> GMQKDSKIYIAGHSGLVGSAILNELKQQGYKNLVFKTHFELDLTNQKAVADFFEREKPEYVILAAAKAGGILANNTYRADFIYQNLMIECNVIHNAYLHKVKKLLFIASTTVYPKNATLPTSEEQMLSGDLEYTNKPYAIAKISGLMLCESYNLQYNTNFIAITPTNLYGNNDKFDLEKSHVLPGILRKMHLAKLLNEKRYEDLLNDLKFDSIEEAKNYLKKFGVDKDNVEIWGSGKPTREFLHSQDLANACLFIMNNIDFKDLKSDNIEIINTHLNIGPHKNITIKELAELIKNIVGFKGKLVFNLNR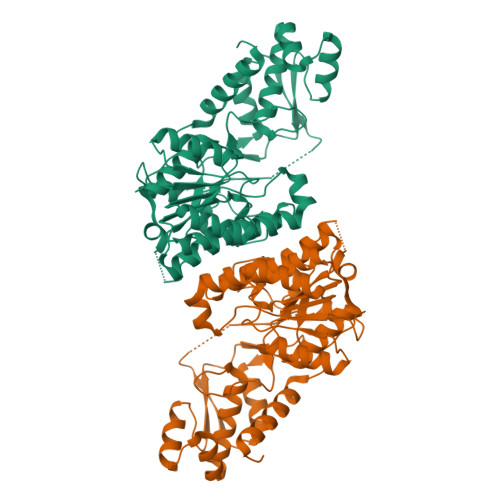PDGAMQKFTDCSKIHSLGWKHKIELEDGIKMMYKWYLKEQNIRQ PENTAETHYLENE GLYCOL MONODECYL ETHER | C20 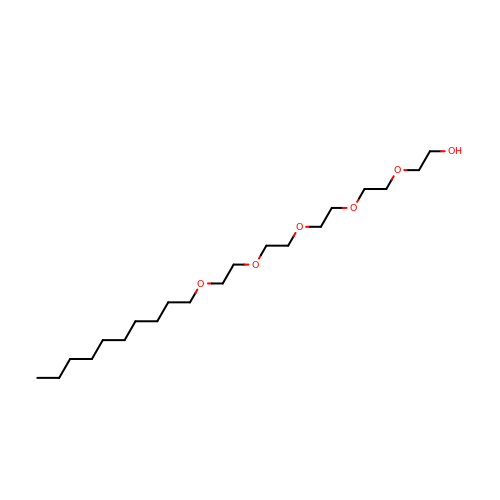H42 O6 | QAXPOSPGRHYIHE-UHFFFAOYSA-N>QRDLSVELGVASNFAILAKAGISSVPDSAILGDIGVSPAAATYITGFGLTQDSSTTYATSPQVTGMIYAADYSTPTPNYLAAAVANAETAYNQAAGFVDPDFLELGAGELRDQTLVPGLYKWTSSVSVPTDLTFEG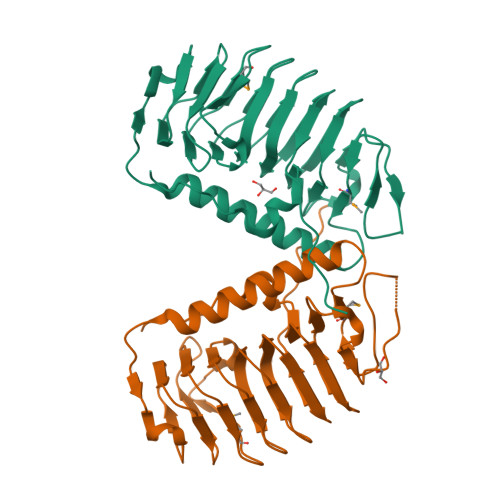NGDATWVFQIAGGLSMADGVAFTLAGGANSTNIAFQVGDDVTVGKGAHFEGVLLAKRFVTLQTGSSLNGRVLSQTEVALQKATVNSPFVPAPEVVQKRSNARQWL[2x]>[2x]MGHHHHHHHHMATLTAKNLAKAYKGRRVVEDVSLTVNSGEIVGLLGPNGAGKTTTFYMVVGIVPRDAGNIIIDDDDISLLPLHARARRGIGYLPQEASIFRRLSVYDNLMAVLQIRDDLSAEQREDRANELMEEFHIEHLRDSM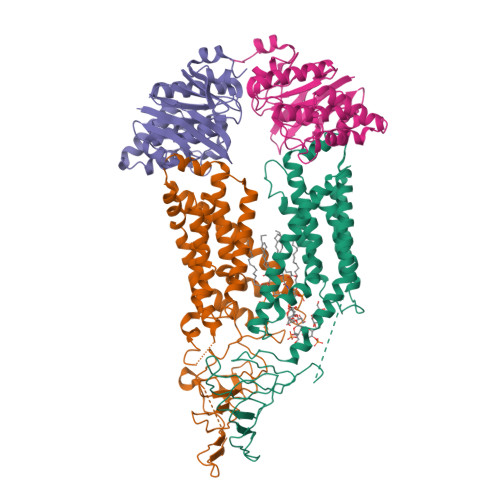GQSLSGGERRRVEIARALAANPKFILLDEPFAGVDPISVIDIKRIIEHLRDSGLGVLITDHNVRETLAVCERAYIVSQGHLIAHGTPTEILQDEHVKRVYLGEDFRL;> MIIIRYLVRETLKSQLAILFILLLIFFCQKLVRILGAAVDGDIPANLVLSLLGLGVPEMAQLILPLSLFLGLLMTLGKLYTESEITVMHACGLSKAVLVKAAMILAVFTAIVAAVNVMWAGPWSSRHQDEVLAEAKANPGMAALAQGQFQQATNGSSVLFIESVDGSDFKDVFLAQIRPKGNARPSVVVADSGHLTQLRDGSQVVTLNQGTRFEGTALLRDFRITDFQDYQAIIGHQAVALDPNDTDQMDMRTLWNTDTDRARAELNWRITLVFTVFMMALMVVPLSVVNPRQGRVLSMLPAMLLYLLFFLIQTSLKSNGGKGKLDPTLWMWTVNLIYLALAIVLNLWDTVPVRRLRASFSRKGAV;> MQPFGVLDRYIGKTIFTTIMMTLFMLVSLSGIIKFVDQLKKAGQGSYDALGAGMYTLLSVPKDVQIFFPMAALLGALLGLGMLAQRSELVVMQASGFTRMQVALSVMKTAIPLVLLTMAIGEWVAPQGEQMARNYRAQAMYGGSLLSTQQGLWAKDGNNFVYIERVKGDEELGGISIYAFNENRRLQSVRYAATAKFDPEHKVWRLSQVDESDLTNPKQITGSQTVSGTWKTNLTPDKLGVVALDPDALSISGLHNYVKYLKSSGQDAGRYQLNMWSKIFQPLSVAVMMLMALSFIFGPLRSVPMGVRVVTGISFGFVFYVLDQIFGPLTLVYGIPPIIGALLPSASFFLISLWLLMRKS ALX5407 | C24 H24 F N O3 | 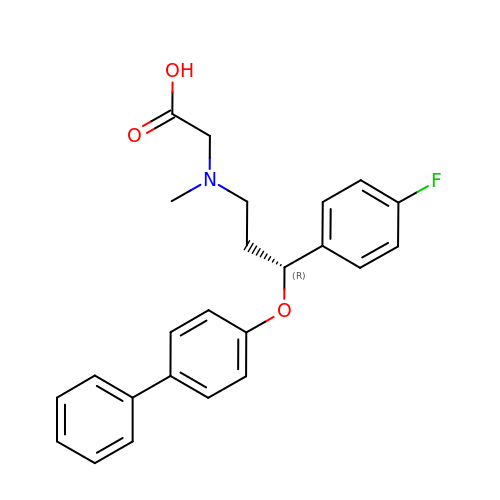FDORQEIHOKEJNX-HSZRJFAPSA-N> MSSSHKSWNSIYEFTVKDINGVDVSLEKYRGHVCLIVNVACKCGATDKNYRQLQEMHTRLVGKGLRILAFPCNQFGGQEPWAEAEIKKFVTEKYGVQFDMFSKIKVNGSDADDLYKFLKSRQHGTLTNNIKW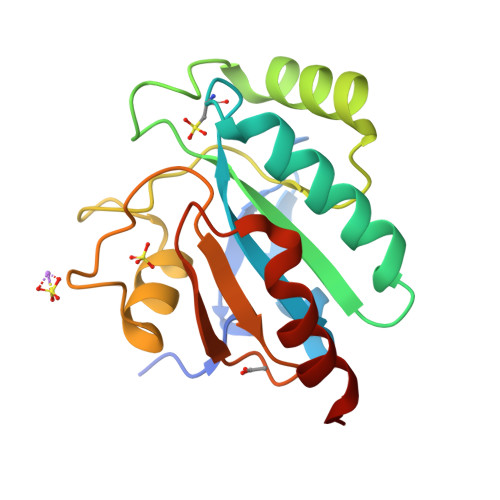NFSKFLVDRQGQPVKRYSPTTAPYDIEGDIMELLEKK> MSKKKFVIVSILTILLVQAIYFVEKYHTSEDKSTSNTSSTPPQTTLSTTKVLKIRYPDDGEWPGAPIDKDGDGNPEFYIEINLWNILNATGFAEMTYNLTSGVLHYVQQLDNIVLRDRSNWVHGYPEIFYGNKPWNANYATDGPIPLPSKVSNLTDFYLTISYKLEPKNGLPINFAIESWLTREAWRTTGINSDEQAVMIWIYYDGLQPAGSKVKEIVVPIIVNGTPVNATFEVWKANIGWEYVAFRIKTPIKE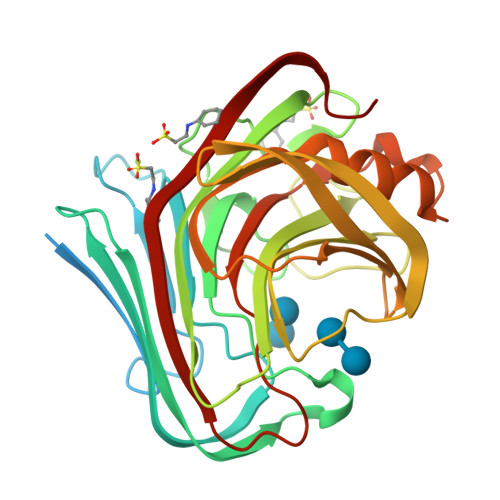GTVTIPYGAFISVAANISSLPNYTELYLEDVEIGTEFGTPSTTSAHLEWWITNITLTPLDRPLIS> GELRVGLEESELWLRFKELTNEMIVTKNGRRMFPVLKVNVSGLDPNAMYSFLLDFVAADNHRWKYVNGEWVPGGKPEPQAPSCVYIH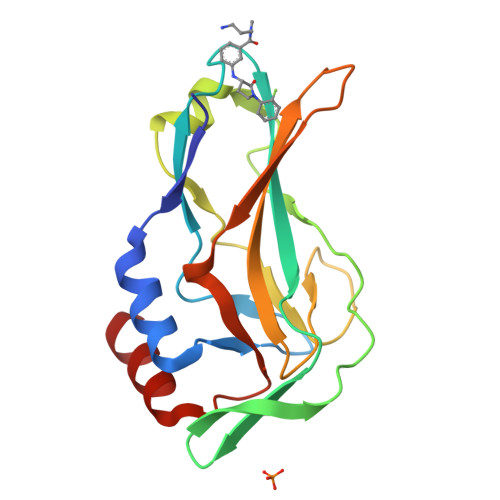PDSPNFGAHWMKAPVSFSKVKLTNKLNGGGQIMLNSLHKYEPRIHIVRVGDPQRMITSHCFPETQFIAVTAYQNEEITALKIKYN> MVEKGKMVKISYDGYVDGKLFDTTNEELAKKEGIYNPAMIYGPVAIFAGEGQVLPGLDEAILEMDVGEEREVVLPPEKAFGKRDPSKIKLIPLSEFTKRGIKPIKGLTITIDGIPGKIVSINSGRVLVDFNHELAGKEVKYRIKIEEVVDDKKNIVKEIVKMYVPRLSDVKVTIRNGTVKIELPEFAPFIPNIQT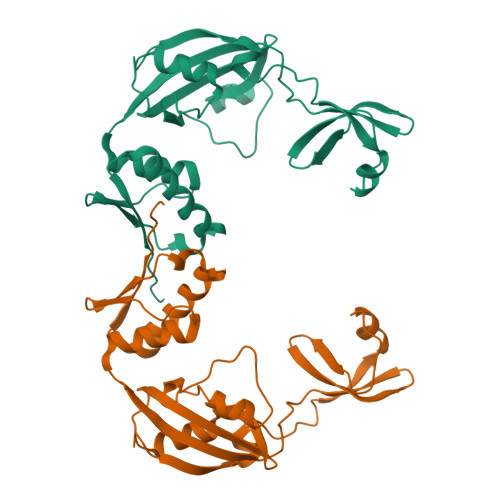AKMAIANEILKRLEDAEKVSFVETFERKKETKEENK> TTHFTVADRWGNVVSYTTTIEQLFGTGIMVPDYGVILNNELTDFDAIPGGAN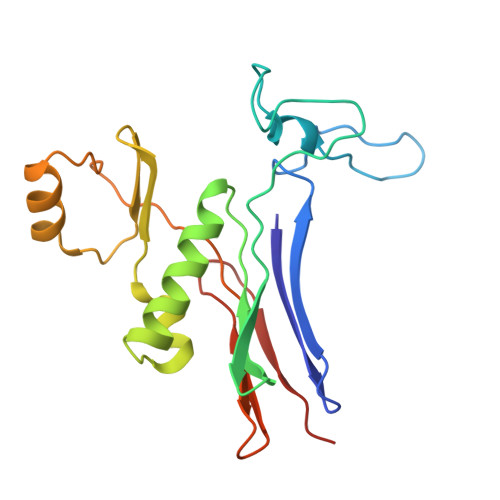EVQPNKRPLSSMTPTILFKDDKPVLTVGSPGGATIISSVLQTILYHIEYGMELKAAVEEPRIYTNSMSSYRYEDGVPKDVLSKLNGMGHKFGTSPVDIGNVQSISIDHENGTFKGVADSSRNGAAIGINLKRK>[2x]PNKTVQFSLYYFGNYESEFSHDKYNLLFAGAKYADQHGFTAVWIPERHFHAFGGFSPNPSVIAAAIARETKQIQIRSGSVVLPLHH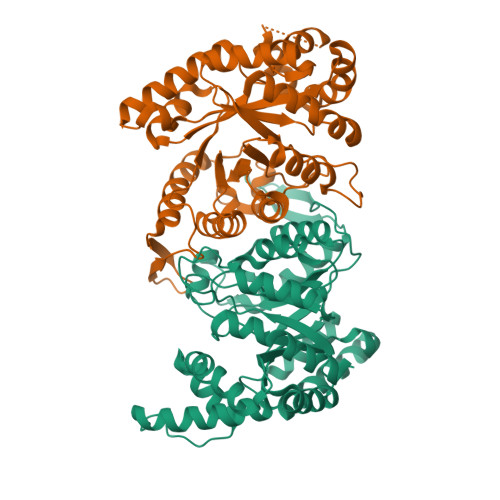PIRVVEEWSVVDNLSQGRVGISFASGWNPNDFALAPQSFGNHRELMFQGIETVRKLWRGEFIQVQNGVGKSISVQAFPRPMQAELPDWITVVNNPETYIKAGEMGSGVLTNLMGQSIEDLAENIALYRESLEKHGYNPASGKVTVLLHTFVGQDLEQTREIARQPLCDYLKSSVALFQNLVKSQGLQVDFDQMTADDQDYILSAAYNRYVQSSALIGTPASCAEVIAKLQAIGVDEVACLIDFGVNTPAVVESLPDLNALRELCQPKTGEQEKEPS> MDYKDDDDKESEMLQSPLLGLGEEDEADLTDWNLPLAFMKKRHCEKIEGSKSLAQSWRMKDRMKTVSVALVLCLNVGVDPPDVVKTTPCARLECWIDPLSMGPQKALETIGANLQKQYENWQPRARYKQSLDPTVDEVKKLCTSLRRNAKEERVLFHYNGHGVPRPTVNGEVWVFNKNYTQYIPLSIYDLQTWMGSPSIFVYDCSNAGLIVKSFKQFALQREQELEVAAINPNHPLAQMPLPPSMKNCIQLAACEATELLPMIPDLPADLFTSCLTTPIKIALRWFCMQKCVSLVPGVTLDLIEKIPGRLNDRRTPLGELNWIFTAITDTIAWNVLPRDLFQKLFRQDLLVASLFRNFLLAERIMRSYNCTPVSSPRLPPTYMHAMWQAWDLAVDICLSQLPTIIEEGTAFRHSPFFAEQLTAFQVWLTMGVENRNPPEQLPIVLQVLLSQVHRLRALDLLGRFLDLGPWAVSLALSVGIFPYVLKLLQSSARELRPLLVFIWAKILAVDSSCQADLVKDNGHKYFLSVLADPYMPAEHRTMTAFILAVIVNSYHTGQEACLQGNLIAICLEQLNDPHPLLRQWVAICLGRIWQNFDSARWCGVRDSAHEKLYSLLSDPIPEVRCAAVFALGTFVGNSAERTDHSTTIDHNVAMMLAQLVSDGSPMVRKELVVALSHLVVQYESNFCTVALQFIEEEKNYALPSPATTEGGSLTPVRDSPCTPRLRSVSSYGNIRAVATARSLNKSLQNLSLTEESGGAVAFSPGNLSTSSSASSTLGSPENEEHILSFETIDKMRRASSYSSLNSLIGVSFNSVYTQIWRVLLHLAADPYPEVSDVAMKVLNSIAYKATVNARPQRVLDTSSLTQSAPASPTNKGVHIHQAGGSPPASSTSSSSLTNDVAKQPVSRDLPSGRPGTTGPAGAQYTPHSHQFPRTRKMFDKGPEQTADDADDAAGHKSFISATVQTGFCDWSARYFAQPVMKIPEEHDLESQIRKEREWRFLRNSRVRRQAQQVIQKGITRLDDQIFLNRNPGVPSVVKFHPFTPCIAVADKDSICFWDWEKGEKLDYFHNGNPRYTRVTAMEYLNGQDCSLLLTATDDGAIRVWKNFADLEKNPEMVTAWQGLSDMLPTTRGAGMVVDWEQETGLLMSSGDVRIVRIWDTDREMKVQDIPTGADSCVTSLSCDSHRSLIVAGLGDGSIRVYDRRMALSECRVMTYREHTAWVVKASLQKRPDGHIVSVSVNGDVRIFDPRMPESVNV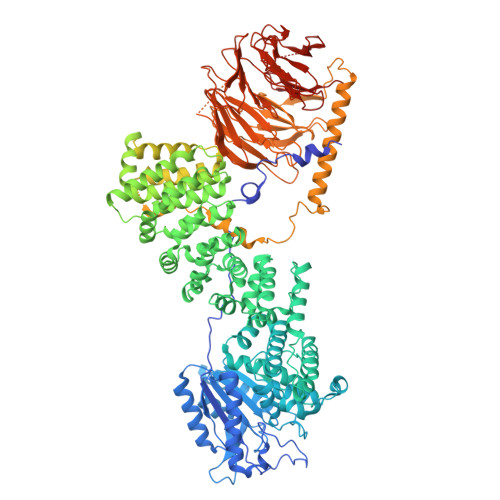LQIVKGLTALDIHPQADLIACGSVNQFTAIYNSSGELINNIKYYDGFMGQRVGAISCLAFHPHWPHLAVGSNDYYISVYSVEKRVR>SNAMKNIKMGMIGLGSIAQKAYLPILTKSERFEFVGAFTPNKVKREKICSDYRIMPFDSIESLAKKCDCIFLHSSTETHYEIIKILLNLGVHVYVDKPLASTVSQGEELIELSTKKNLNLMVGFNRRFCPMYKEIKNNATEIVSINICKHGLNSLRNVRFDSTLIDDYIHVIDTALWLANEDVEISGEDLFLTDNKNLIFVSHKLKGKNFSINTSMHRDSGTKLEQVEILSKGKIQRVKNLNVLEIEEGGNLTLKQSGAWVNILKQKGFEDISNHFIDCIENNIKPAINGEECIKAQRLLEKIINSVK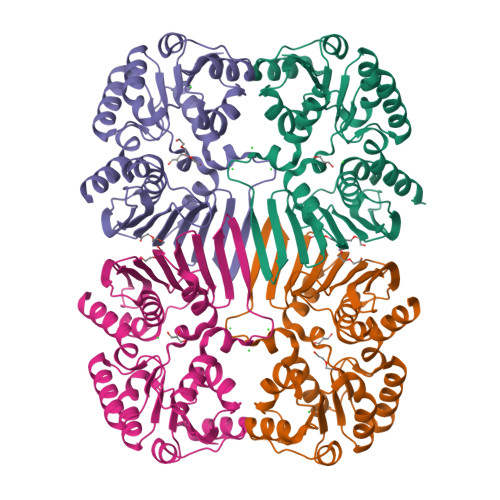[4x]>[12x]YFQNSAMTKTKFEKVLLIVNPKAGQGDLHTNLTKIVPPLAAAFPDLHILHTKEQGDATKYCQEFASKVDLIIVFGGDGTVFECTNGLAPLEIRPTLAIIPGGTCNDFSRTLGVPQNIAEAAKLITKEHVKPVDVAKANGQHFLNFWGIGLVSEVSNNIDAEEKAKLGKIGYYLSTIRTVKNAETFPVKITY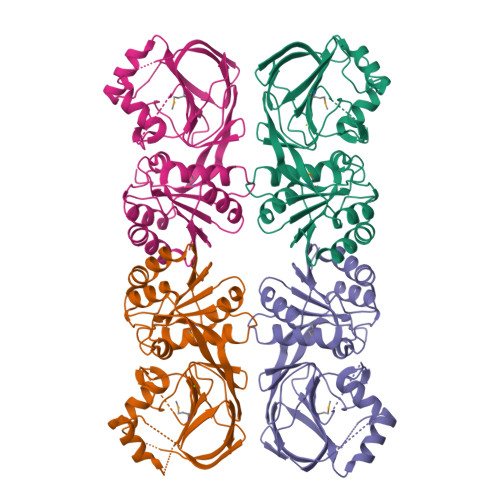DGQVYEDEAVLVMVGNGEYLGGIPSFIPNVKCDDGTLDIFVVKSTGIQAFKDYIGKKLFEDSNENDIFHVKAKSIHIETEEEKEVDTDGESSLHTPCQIELLQGHFTMIYNPAVV> MFSAFRDTASIGFSDTHQDEKTLRFLKKQISQFIKHLKEYYPNNELTKKLVMKYSDVQLL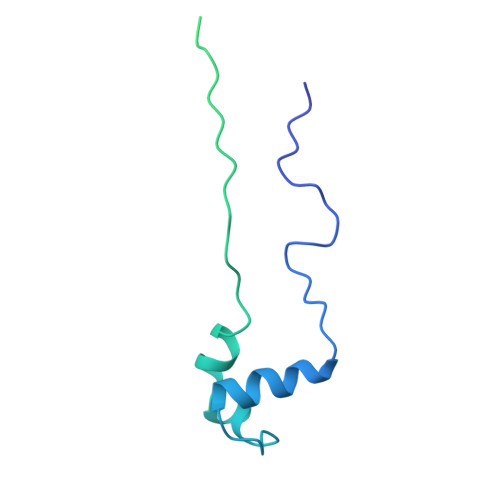PYTKGATKDTYTSGLFDHTTGVIKIAPRDGLGNVRDEQSLNKSICHELAHGTRVKYPGESSHSDEWKDAWKTFLKIAADELGWKIEVPCSSVSFYGLTKDDCENCVWDQDPETCPKTAKLA>[2x]MGSSHHHHHHSSGLVPPGSMSEQYWRFKLMTEGGCNQNEATRLITVLKRKLKPFPEESINKLFENDNFCNRLSSYMAYGFGAAEEWIKKQQILSNIQPLTSEQRVDITPEKDTVSDNKPNIFGAAITFGKSPVVKLLKQNAREICESILMDEPNLKQVEYIFRLLALQVQETYSGEQAEKLYECIRDKKPIPSKFEEILLPIVNRIKENHTEILNESKRNHLGVTIQLNDPYSFSTKNSFCIWFSNNPNSAMPKKIKDILEERAKQNAPGVTKLVYSRACLTKKENTNFVQWAKENGITLLDFDELKCQGEDLEL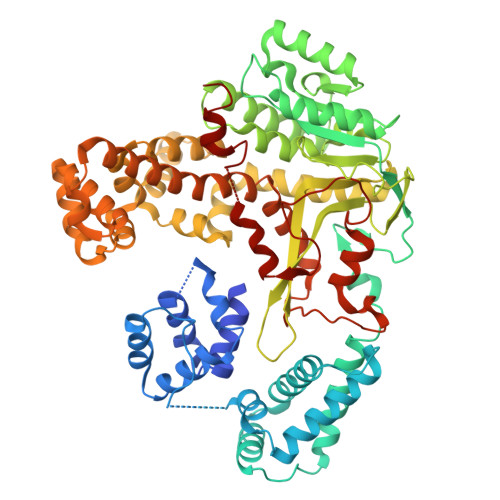WNLAQAELKAMREGKGGNPAAASDLVRWISGVIGDVPIAYVDADMPMLTGNKSIKSEEVYAGHPVLLNMGSALVKDGVNLPMENVAFNTDIINFTGECKDRSIAIKRIAQSLIGNYLHVTERISKSGNPELKRLGLMPGYHQLLKDCEENNNKLSLPMLRKALTQAHSNLSSYVRFIGVQRFAEMVGAPEDAPLFQEALQQGNTIVLTNALVAYLVHGMDNVSRLNSSEKENLIKKYLGTQLSLLYKPLVMEFSGPCAVTREILPLLPTGEPTRYIENLKQPDAQILRVLQTHACVAGKTNFTSDNIPNWITSSEEVERTQSLRTDGLSWMPSEQARLSK> DRHHHHHHGSVTQRTFKLDYSRDRFLKDGQPFRYISGSIHYFRIPRFYWEDRLLKMKMAGLNAIQM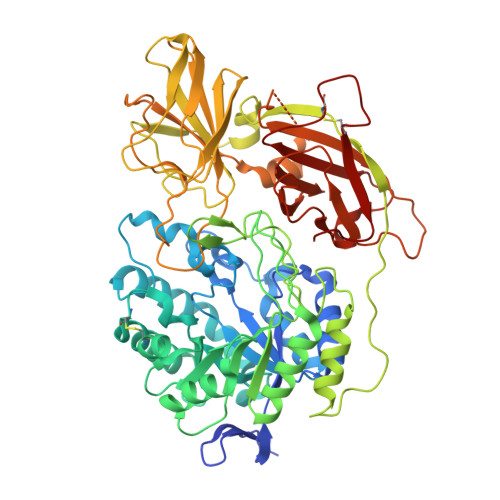YVPWNFHEPQPGQYEFSGDRDVEHFIQLAHELGLLVILRPGPYICAEWDMGGLPAWLLEKQSIVLRSSDPDYLVAVDKWLAVLLPKMKPLLYQNGGPIITVQVENEYGSYFACDYDYLRFLVHRFRYHLGNDVILFTTDGASEKMLKCGTLQDLYATVDFGTGNNITQAFLVQRKFEPKGPLINSEFYTGWLDHWGKPHSTVKTKTLATSLYNLLARGANVNLYMFIGGTNFAYWNGANTPYEPQPTSYDYDAPLSEAGDLTKKYFALREVIQMFKEVPEGPIPPSTPKFAYGKVALRKFKTVAEALGILCPNGPVKSLYPLTFTQVKQYFGYVLYRTTLPQDCSNPKPIFSSPFNGVRDRAYVSVDGVPQGILDRNLMTALNIQGKAGATLDILVENMGRVNYGRFINDFKGLISNMTINSTVLTNWTVFPLDTEAMVRNHLWGREASDGGHLDGRSTSNSSDLILPTFYVGNFSIPSGIPDLPQDTFIQFPGWSKGQVWINGFNLGRYWPTMGPQKTLFVPRNILTTSAPNNITVLELEFAPCSEGTPELCTVEFVDTPVIS>GLKQKIVIKVAMEGNNCRSKAMALVASTGGVDSVALVGDLRDKIEVVGYGIDPIKLISALRKKVGDAELLQVSQAKKD[4x];>METGNKYIEKRAIDLSRERDPNFFDNPGIPVPECFWFMFKNNVRQDDGTC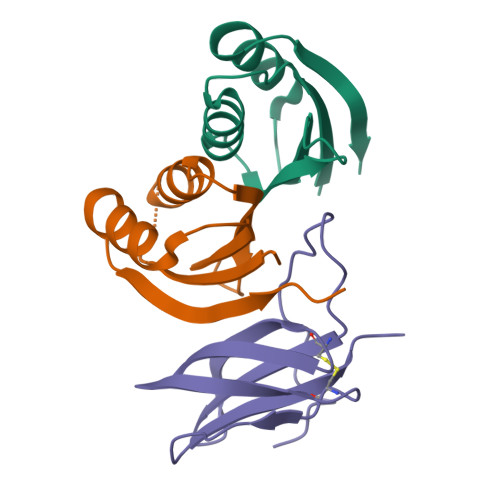YSSWKMDMKVGPNWVHIKSDDNCNLSGDFPPGWIVLGKKRPGF[2x]> GRARAVENQYSF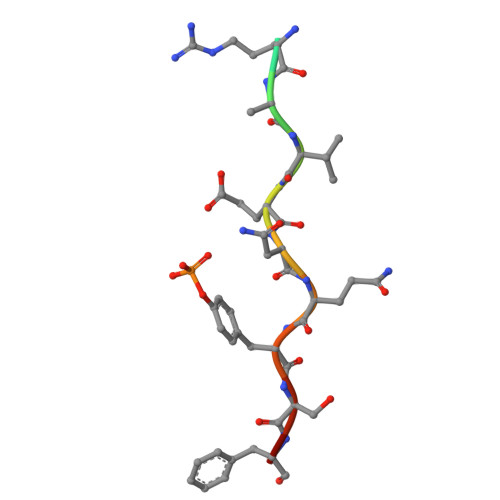Y> AALPQDEKLITGQLDNGLRYMIYPHAHPKDQVNLWLQIHTGSLQEEDNELGVAHFVEHMMFNGTKTWPGNKVIETFESMGLRFGRDVNAYTSYDETVYQVSLPTTQKQNLQQVMAIFSEWSNAATFEKLEVDAERGVITEEWRAHQDAKWRTSQARRPFLLANTRNLDREPIGLMDTVATVTPAQLRQFYQRWYQPNNMTFIVVGDIDSKEALALIKDNLSKLPANKAAENRVWPTKAENHLRFNIINDKENRVNGIALYYRLPMVQVNDEQSFIEQAEWSMLVQLFNQRLQERIQSGELKTISGGTARSVKIAPDYQSLFFRVNARDDNMQ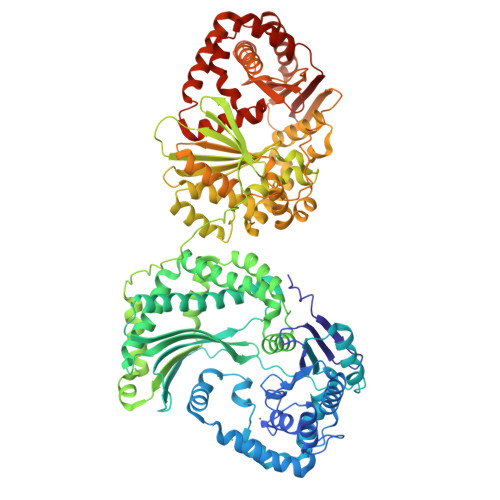DAANALMAELATIDQHGFSAEELDDVKSTRLTWLKNAVDQQAERDLRMLTSRLASSSLNNTPFLSPEETYQLSKRLWQQITVQSLAEKWQQLRKNQDAFWEQMVNNEVAAKKALSPAAILALEKEYANKKLAAYVFPGRNLSLTVDADPQAEISSKETLAENLTSLTLSNGARVILAKSAGEEQKLQIIAVSNKGDLSFPAQQKSLIALANKAVSGSGVGELSSSSLKRWSAENSVTMSSKVSGMNTLLSVSARTNNPEPGFQLINQRITHSTINDNIWASLQNAQIQALKTLDQRPAEKFAQQMYETRYADDRTKLLQENQIAQFTAADALAADRQLFSSPADITFVIVGNVAEDKLVALITRYLGSIKHSDSPLAAGKPLTRATDNASVTVKEQNEPVAQVSQWKRYDSRTPVNLPTRMALDAFNVALAKDLRVNIREQASGAYSVSSRLSVDPQAKDISHLLAFTCQPERHDELLTLANEVMVKRLAKGISEQELNEYQQNVQRSLDIQQRSVQQLANTIVNSLIQYDDPAAWTEQEQLLKQMTVENVNTAVKQYLSHPVNTYTGVLLPKLEHHHHHH>MGHHHHHHEFMLKNDDFVIAKNQLGNIVPNSVGVIRAVNGKSAMVLFIGLNELKRVDFSELEAIDIYRTGKGYDKKICNICHILKNTDGFEINQTDAKGRKTTRPSCRECRKNIDGVKLSSTEKKKMDEIAPPKGSVFTCPICEKRSIVGVTANLVHDHNHDTGWGREWICDSCNTGL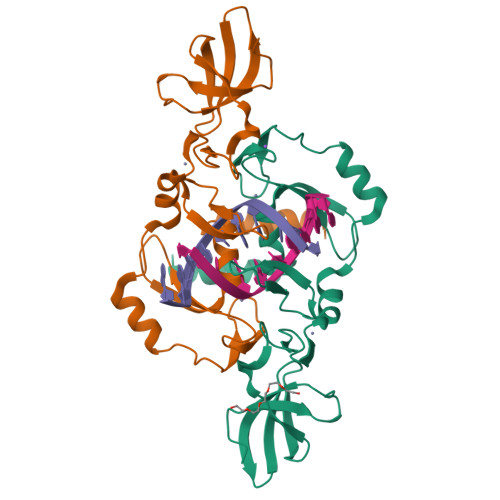GRFKDNPKFLEKVIEYLKKYEK[2x]> APFTGPILTVEEMSNSRFPIPLEKLYTGPSGAFVVQPQNGRCTTDGVLLGTTQLSAVNICTFRGDVTGVAGSHDYIMNLASQNWNNYDPTEEIPAPLGTPDFVGKIQGMLTQTTREDGSTRAHKATVSTGSVHFTPKLGSVQYTTDTNNDLQTGQNTKFTPVGVIQDGNHQNEPGGWVLPNYSGRTGHNVHLAPAVAPTFPGEQLLFFRSTMPGCSGYPNMNLDCLLPQEWVQHFYQEAAPAQSDVALLRFVNPDTG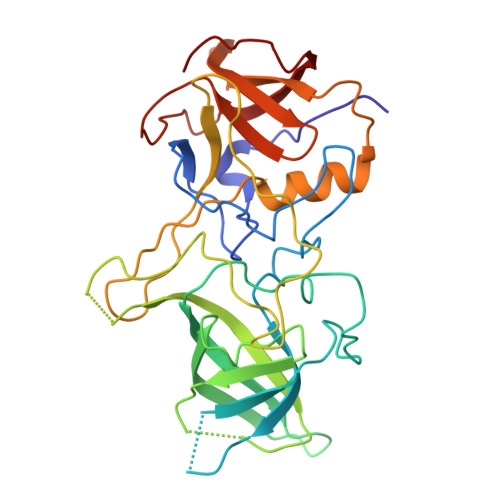RVLFECKLHKSGYVTVAHTGPHDLVIPPNGYFRFDSWVNQFYTLAPM>CGIVGIAGVMPVNQSIYDALTVLQHRGQDAAGIITIDANNCFRLRKANGLVSDVFEARHMQRLQGNMGIGHVRYPTAGSSSASEAQPFYVNSPYGITLAHNGNLTNAHELRKKLFEEKRRHINTTSDSEILLNIFASELDNFRHYPLEADNIFAAIAATNRLIRGAYACVAMIIGHGMVAFRDPNGIRPLVLGKRDIDENRTEYMVASESVALDTLGFDFLRDVAPGEAIYITEEGQLFTRQCADNPVSNPCLFEYVYFARPDSFIDKISVYSARVNMGTKLGEKIAREWEDLDIDVVIPIPETSCDIALEIARILGKPYRQGFVKNRYVGRTFIMPGQQLRRKSVRRKLNANRAEFRDKNVLLVDDSIVRGTTSEQIIEMAREAGAKKVYLASAAPEIRFPNVYGIDMPSATELIAHGREVDEIRQIIGADGLIF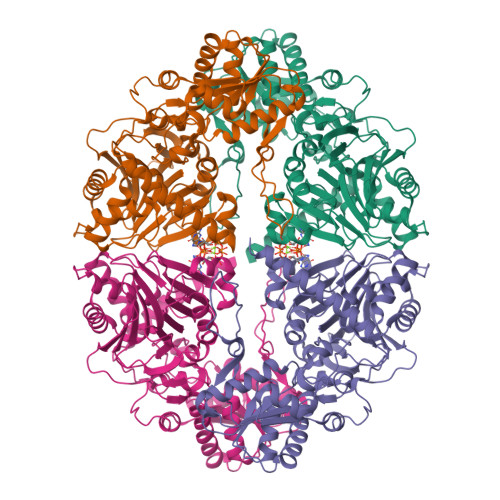QDLNDLIDAVRAENPDIQQFECSVFNGVYVTKDVDQGYLDFLDTLRNDDAKAVQRQNEVENL[4x]> GGPNLFVALYDFESRTENTLSITKGEKLRVLGYNHNGEWCEAQTKNGQGWVPSNYITPVN

The Src homology 3 (SH3) domain is a ∼60-residue modular domain that consists of two antiparallel β-sheets orthogonally packed to form a single hydrophobic core. This domain is present in many proteins and regulates critical cellular pathways by recognizing polyproline-rich motifs (PRMs; Kurochkina & Guha, 2013). Three-dimensional domain swapping (3D-DS) is a mechanism by which some proteins can oligomerize by exchanging identical domains or structural elements between monomers. In previous work, the 3D-DS of the c-Src SH3 domain has been characterized and its dependence on experimental conditions has been described. This work explores the role of the hinge-loop composition by interchanging residues in the RT and n-Src loops between two SH3 domains: one being the c-Src SH3 domain, where 3D-DS has been described, and the other being the Abl SH3 domain, where 3D-DS has not been described to date.

However, the interchange of one or two loops within the Abl SH3 domain produces a noticeable reduction in its stability but does not promote the formation of 3D domain-swapped oligomers. Conversely, replacing the RT and n-Src loop residues in the Abl_Src chimeras with those from the c-Src SH3 domain results in destabilization under identical denaturing conditions. In this way, the ΔG values are the same for the WT and Abl_Src-RT, but the Abl_Src-nSrc and Abl_Src-2 chimeras show a noticeable loss of stability. Similar to the results from chemical denaturation, these data point to lower stability in those chimeras where the n-Src loop was exchanged, whereas the RT loop has a minimal effect on stability. Although the conformation is slightly different in the RT loop, the hydrogen bonds are conserved. In the n-Src loop, there are significant differences between the WT protein and Abl_Src-nSrc, but also with the Abl_Src-RT and Abl_Src-2 chimeras. However, Src_Abl-nSrc shows an ordered distal loop in most of the molecules in the asymmetric unit and this chimera does not form the intertwined dimer. The same behaviour can be observed in the Abl_Src chimeras, where the distal loop shows low B factors. Indeed, even though the Abl_Src chimeras are less stable, this reduction in stability does not allow formation of the intertwined dimer.> ASGTSLSAAIHRTQLWFHGRISREESQRLIGQQGLVDGLFLVRESQRNPQGFVLSLCHLQKVKHYLILPSEEEGRLYFSMDD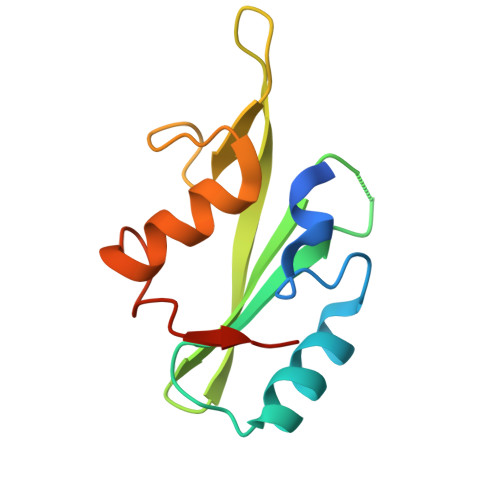GQTRFTDLLQLVEFHQLNRGILPCLLRHCCTRVAL>MQKTLEVWIMPNSPQPAEDFKALVAPFEKAHGVEVKVTVLDWGVAWTKITTAATSGV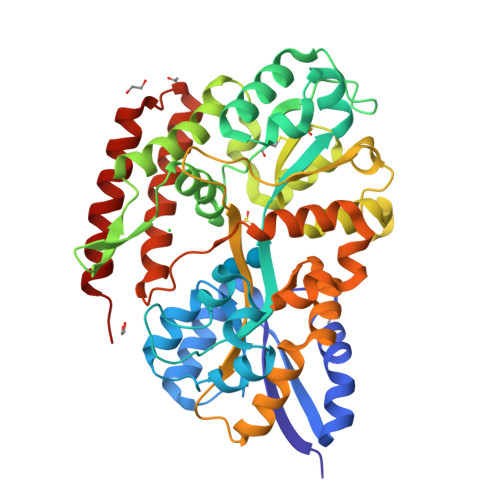GPDLTQLGTTWVGAISAMGVLEPVDDVLEALGGEKAYLPAVWRTTRLEGARQATAVPWFSELRAFYYRTDALKAAGVNPAEMFASWQGFEAGLARLKASSFRDPETKAPLAPLCTPGRTPRTLHNAAPWIWGAGGEIVRQAGGRWQSALNSPESLEGLYFFLSLAQKGYVPAESLEKNTAQIEADFQAGKCAVFASGPWMIQRAQVPEAKGGFAERTAAKNLGVAPYPAGPKGRYTFFGGSNLALFNFSKNKPLAKELLKYLGGPEAQVRYAQMTGMLPALRSAWSDPSFQQNPLLRTFIQAAQFGRTYPSLAGWGGVENLAVQHLGMAWDLVAQGRLTREALKDLMDKASAAINQALRHHHHHH[2x]> GSHMTCWLRGVTATFGRPAEWPGYLSHLCGRSAAMDLGPMRKSYRGDREAFEETHLTSLDPVKQFAAWFEEAVQCPDIGEANAMCLATCTRDGKPSARMLLLKGFGKDGFRFFTNFESRKGKELDSNPFASLVFYWEPLNRQVRVEGPVKKLPEEEAECYFHSRPKSSQIGAVVSHQSSVIPDREYLRKKNEELEQLYQDQEVPKPKSWGGYVLYPQVMEFWQGQTNHLHDRIVFRRGLPTGDSPLGPMTHRGEEDWLYERLAP

The enzyme pyridox(am)ine 5′‐phosphate oxidase (PNPO), whose catalytic action yields PLP, is one of the key players in this pathway. In humans, the different B6 vitamers, introduced with food, are interconverted through a salvage pathway which involves, besides kinases and phosphatases, the enzyme pyridoxine 5′‐phosphate (PNP)/pyridoxamine 5′‐phosphate (PMP) oxidase (PNPO) (di Salvo et al., 2011, 2012). This flavin mononucleotide (FMN)‐dependent enzyme, which produces PLP from PNP or PMP, plays an active role in vitamin B6 homeostasis. In both human and E. coli PNPO, PLP works as a regulator of its own production because it binds at an allosteric site of the enzyme, affecting the binding of substrate at the active site and inhibiting the catalytic activity (Barile et al., 2019, 2021). Mutations in the gene encoding PNPO are responsible for a severe form of neonatal epilepsy.

On the basis of this previous experience, we carried out co‐crystallization attempts with either the wild type or the R225H variant of the human protein and PLP. The R225H variation affects a crucial active site residue involved in substrate binding, but is able to bind PLP at the allosteric site and has allosteric properties (Barile et al., 2020). We obtained crystals with both protein forms; however, PLP was detected only in the active site of the wild type protein, thus a clear indication about the location of the allosteric site was missing. A substantial part of the N‐terminal end is not visible in these structures: the electron density map starts from Glu46 in the R225H and from Ala47 in the wild type structure. PLP binding at the allosteric site of E. coli PNPO results in the disorder of the large structural region made by residues 123–166 and also uncoils a short helix (residues 192–200), which contains Arg197 (corresponding to Arg225 of human PNPO) that plays a crucial role in binding the vitamer substrates at the active site. Our crystallographic analyses and the results concerning the proteolysis of PNPO N‐terminal region indicate that this region of the protein is very flexible.> GPHMASSSGAGAAAAAAAANLNAVRETMDVLLEISRILNTGLDMETLSICVRLCEQGINPEALSSVIKELRKATEALKAA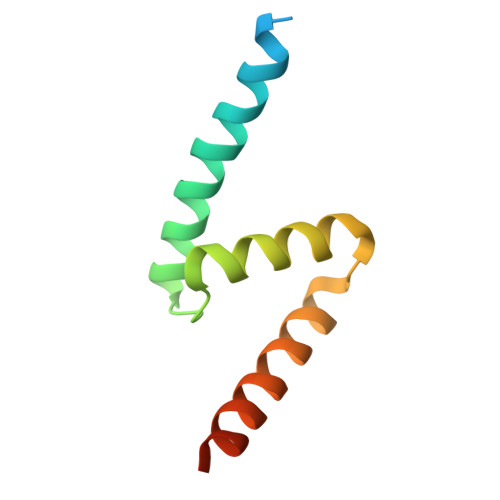ENMTS>MGKIKIGINGFGRIGRLVARVALQSEDVELV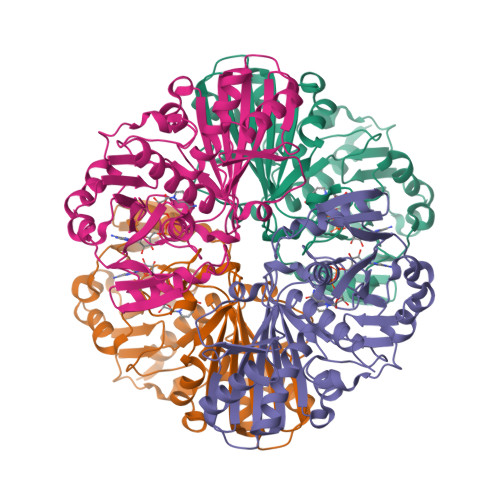AVNDPFITTDYMTYMFKYDTVHGQWKHSDIKIKDSKTLLLGEKPVTVFGIRNPDEIPWAEAGAEYVVESTGVFTDKEKAAAHLKGGAKKVVISAPSKDAPMFVCGVNEDKYTSDIDIVSNASCTTNCLAPLAKVIHDNFGIIEGLMTTVHAITATQKTVDGPSSKDWRGGRAASFNIIPSSTGAAKAVGKVLPDLNGKLTGMSFRVPTVDVSVVDLTVRIEKAASYDAIKSAIKSASEGKLKGIIGYVEEDLVSTDFVGDSRSSIFDAKAGIALNDNFVKLVAWYDNEWGYSNRVIDLIRHMAKTQ[4x]> MTNEQVIELVRVLLGGITTEEISDQTIIFFWTKWKLTYDLDNRPE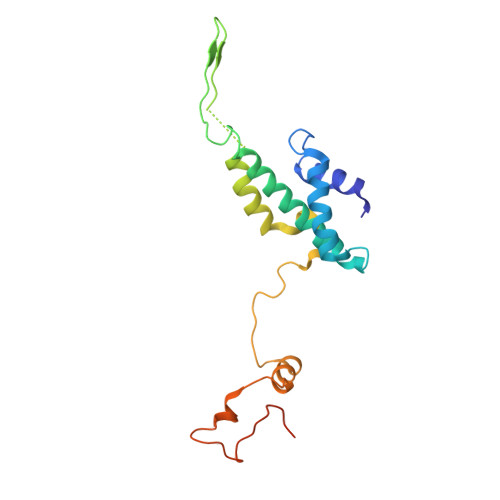KIPAALYNTVVDCVRWLIVQEVSSGNSSIRERFEKIGDETISVKGGSSWESWKDFLDWLELNPDYIDPSLAFNSSLVIIGGVRKDEFFRVKNNPNSYNGFMEQGVYPTPAIPKQSAWPCTAARRSPWMVR>[2x]GAEVRAESIAQPTPINVIFPDPALANAVKTATGKSNVTDAVTQADLDGIATLSAFNTGVTTIEGIQ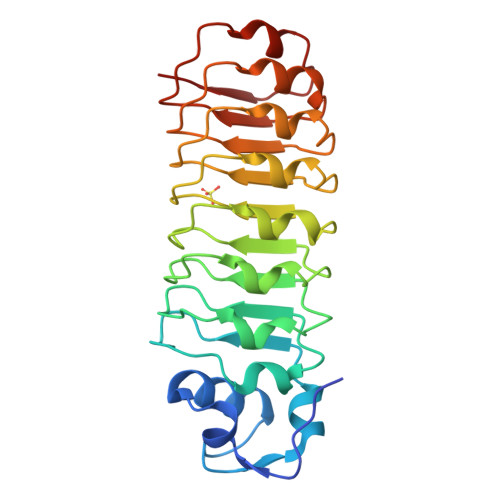YLNNLIGLELKDNQITDLTPLKNLTKITELELSGNPLKNVSAIAGLQSIKTLDLTSTQITDVTPLAGLSNLQVLYLDLNQITNISPLAGLTNLQYLSIGNNQVNDLTPLANLSKLTTLRADDNKISDISPLASLPNLIEVHLKDNQISDVSPLANLSNLFIVTLT>RHMTRYDSLLQALGNTPLVGLQRLSPRWDDGRDGPHVRLWAKLEDRNPTGSIKDRPAVRMIEQAEADGLLRPGATILEPTSGNTGISLAMAARLKGYRLICVMPENTSVERRQLLELYGAQIIFSAAEGGSNTAVATAKELAATNPSWVMLYQYGNPANTDSHYCGTGPELLADLPEITHFVAGLGTTGTLMGTGRFLREHVANVKIVAAEPRYGEGVYALRNMDEGFVPELYDPEILTARYSVGAVDAVRRTRELVHTEGIFAGISTGAVLHAALGVGAGALAAGERADIALVVADAGWKYLSTGAYAGSLDDAETALEGQLWA[2x];> MNVTVSIPTILRPHTGGQKSVSASGDTLGAVISDLEANYSGISERLMDPSSPGKLHRFVNIYVNDEDVRFSGGLATAIADGDSVTIL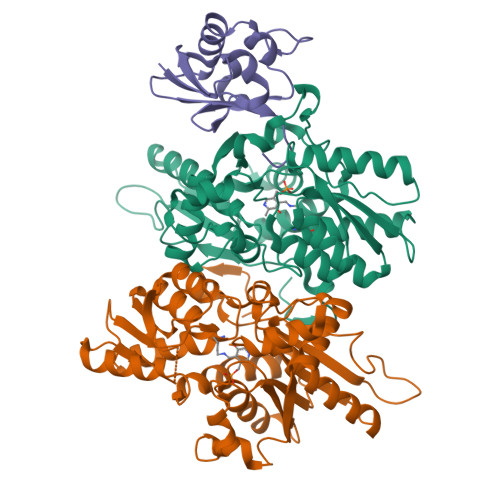PAVAGG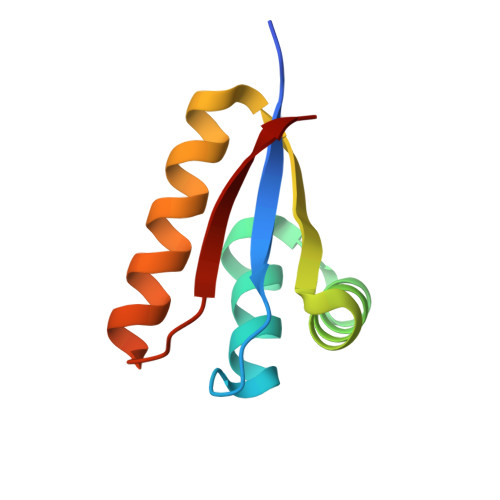>[2x]TQKPSLYRVLILNDDYTPMEFVVYVLERFFNKSREDATRIMLHVHQNGVGVCGVYTYEVAETKVAQVIDSARRHQHPLQCTMEKD> MPYSVGFREADAATSFLRAARSGNLDKALDHLRNGVDINTCNQNGLNGLHLASKEGHVKMVVELLHKEIILETTTKKGNTALHIAALAGQDEVVRELVNYGANVNAQSQKGFTPLYMAAQENHLEVVKFLLENGANQNVATEDGFTPLAVALQQGHENVVAHLINYGTKGKVRLPALHIAARNDDTRTAAVLLQNDPNPDVLSKTGFTPLHIAAHYENLNVAQLLLNRGASVNFTPQNGITPLHIASRRGNVIMVRLLLDRGAQIETKTKDELTPLHCAARNGHVRISEILLDHGAPIQAKTKNGLSPIHMAAQGDHLDCVRLLLQYDAEIDDITLDHLTPLHVAAHCGHHRVAKVLLDKGAKPNSRALNGFTPLHIACKKNHVRVMELLLKTGASIDAVTESGLTPLHVASFMGHLPIVKNLLQRGASPNVSNVKVETPLHMAARAGHTEVAKYLLQNKAKVNAKAKDDQTPLHCAARIGHTNMVKLLLENNANPNLATTAGHTPLHIAAREGHVETVLALLEKEASQACMTKKGFTPLHVAAKYGKVRVAELLLERDAHPNAAGKNGLTPLHVAVHHNNLDIVKLLLPRGGSPHSPAWNGYTPLHIAAKQNQVEVARSLLQYGGSANAESVQGVTPLHLAAQEGHAEMVALLLSKQANGNLGNKSGLTPLHLVAQEGHVPVADVLIKHGVMVDATTRMGYTPLHVASHYGNIKLVKFLLQHQADVNAKTKLGYSPLHQAAQQGHTDIVTLLLKNGASPNEVSSDGTTPLAIAKRLGYISVTDVLKVVTDETSFVLVSDKHRMSFPETVDEILDVSEDEGEELISFKAERRDSRDVDEEKELLDFVPKLDQVVESPAIPRIPCAMPETVVIRSEEQEQASKEYDEDSLIPSSPATETSDNISPVASPVHTGFLVSFMVDARGGSMRGSRHNGLRVVIPPRTCAAPTRITCRLVKPQKLSTPPPLAEEEGLASRIIALGPTGAQFLSPVIVEIPHFASHGRGDRELVVLRSENGSVWKEHRSRYGESYLDQILNGMDEELGSLEELEKKRVCRIITTDFPLYFVIMSRLCQDYDTIGPEGGSLKSKLVPLVQATFPENAVTKRVKLALQAQPVPDELVTKLLGNQATFSPIVTVEPRRRKFHRPIGLRIPLPPSWTDNPRDSGEGDTTSLRLLCSVIGGTDQAQWEDITGTTKLVYANECANFTTNVSARFWLSDCPRTAEAVNFATLLYKELTAVPYMAKFVIFAKMNDPREGRLRCYCMTDDKVDKTLEQHENFVEVARSRDIEVLEGMSLFAELSGNLVPVKKAAQQRSFHFQSFRENRLAMPVKVRDSSREPGGSLSF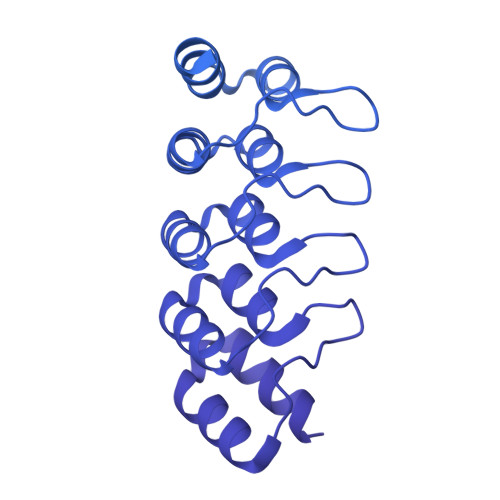LRKAMKYEDTQHILCHLNITMPPCAKGSGAEDRRRTPTPLALRYSILSESTPGSLSGTEQAEMKMAVISEHLGLSWAELARELQFSVEDINRIRVENPNSLLEQSVALLNLWVIREGQNANMENLYTALQSIDRGEIVNMLEGSGRQSRNLKPDRRHTDRDYSLSPSQMNGYSSLQDELLSPASLGCALSSPLRADQYWNEVAVLDAIPLAATEHDTMLEMSDMQVWSAGLTPSLVTAEDSSLECSKAEDSDATGHEWKLEGALSEEPRGPELGSLELVEDDTVDSDATNGLIDLLEQEEGQRSEEKLPGSKRQDDATGAGQDSENEVSLVSGHQRGQARITHSPTVSQVTERSQDRLQDWDADGSIVSYLQDAAQGSWQEEVTQGPHSFQGTSTMTEGLEPGGSQEYEKVLVSVSEHTWTEQPEAESSQADRDRRQQGQEEQVQEAKNTFTQVVQGNEFQNIPGEQVTEEQFTDEQGNIVTKKIIRKVVRQIDLSSADAAQEHEEVTVEGPLEDPSELEVDIDYFMKHSKDHTSTPNP>[2x]TDTTLPPDDSLDRIEPVDIEQEMQRSYIDYAMSVIVGRALPEVRDGLKPVHRRVLYAMFDSGFRPDRSHAKSARSVAETMGNYHPHGDASIYDSLVRMAQPWSLRYPLVDGQGNFGSPGNDPPAAMRYTEARLTPLAMEMLREIDEETVDFIPNYDGRVQEPTVLPSRFPNLLANGSGGIAVG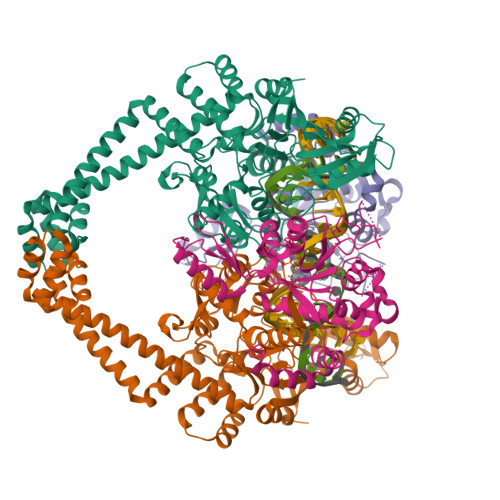MATNIPPHNLRELADAVFWALENHDADEEETLAAVMGRVKGPDFPTAGLIVGSQGTADAYKTGRGSIRMRGVVEVEEDSRGRTSLVITELPYQVNHDNFITSIAEQVRDGKLAGISNIEDQSSDRVGLRIVIEIKRDAVAKVVINNLYKHTQLQTSFGANMLAIVDGVPRTLRLDQLIRYYVDHQLDVIVRRTTYRLRKANERAHILRGLVKALDALDEVIALIRASETVDIARAGLIELLDIDEIQAQAILDMQLRRLAALERQRIIDDLAKIEAEIADLEDILAKPERQRGIVRDELAEIVDRHGDDRRTRIIAIGSG;>[2x]SNALVRRKSATDIGGLPGKLADCRSTDPRKSELYVVEGDSAGGSAKSGRDSMFQAILPLRGKIINVEKARIDRVLKNTEVQAIITALGTGIHDEFDIGKLRYHKIVLMADADVDGQHISTLLLTLLFRFMRPLIENGHVFLAQPPLYKLKWQRSDPEFAYSDRERDGLLEAGLKAGKKINKEDGIQRYKGLGEMDAKELWETTMDPSVRVLRQVTLDDAAAADELFSILMGEDVDARRSFITRNAKDVRFLDV Mimivirus is the prototype of the Mimiviridae family of giant dsDNA viruses. Little is known about the organization of the 1.2 Mb genome inside the membrane-limited nucleoid filling the ~0.5 µm icosahedral capsids. Cryo-electron microscopy, cryo-electron tomography, and proteomics revealed that it is encased into a ~30-nm diameter helical protein shell surprisingly composed of two GMC-type oxidoreductases, which also form the glycosylated fibrils decorating the capsid. The genome is arranged in 5- or 6-start left-handed super-helices, with each DNA-strand lining the central channel.

An additional step of refinement focused on the asymmetric unit further improved the local resolution to 3.3 Å as indicated by the corresponding FSC. In the 3.3-Å resolution map of the asymmetric unit, most side chains and notably the FAD cofactor are accommodated by density suggesting that the oxidoreductase enzyme could be active. The N-terminal chain, being more disordered than the rest of the structure, it is absent in the focused refined map, and also absent in the Cl3a map of the relaxed helix, suggesting that a break of the disulfide bridge could be involved in the observed unwinding process.

>MAHRSRCNCNDTSNSNGSQHGINLPLRKIDTYDPCVNCRVKPHLCPKPHPCPKPENLEADIVIIGAGAAGCVLAYYLTKFSDLKIILLEAGHTHFNDPVVTDPMGFFGKYNPPNENIRMSQNPSYAWQPALEPDTGAYSMRNVVAHGLAVGGSTAINQLNYIVGGRTVFDNDWPTGWKYDDIKKYFRRVLADISPIRDGTKVNLTNTILESMRVLADQQVSSGVPVDFLINKATGGLPNIEQTYQGAPIVNLNDYEGINSVCGFKSYYVGVNQLSDGSYIRKYAGNTYLNSYYVDSNGFGIGKFSNLRVISDAVVDRIHFEGQRAVSVTYIDKKGNLHSVKVHKEVEICSGSFFTPTILQRSGIGDFSYLSSIGVPDLVYNNPLVGQGLRNHYSPITQVSVTGPDAAAFLSNTAAGPTNMSFRGAGMLGYHKLEPNKPSNAGSVTYRKYELLVTGGVAISADQQYLSGISSSTGNYFALIADDIRFAPVGYIKIGTPNFPRDTPKIFFNTFVNYTPTTDPADQQWPVAQKTLAPLISALLGYDAIYQIVQQMKVVAVNAGFNVTLQMAYPPNDLLVELHNGLNTYGINWWHYFVPSLVNDDTPAGKLFASTLSKLSYYPRSGAHLDSHQSCSCSIGGTVDTELKVIGVENVRVTDLSAAPHPPGGNTWCTAAMIGARATDLILGKPLVANLPPEDVPVFTTS[2x]> TIGSEFQNDIPDLYSVFKDYFPIGVAVDPSRLNDTDPHAQLTAKHFNMLTAENAMKPESLEPEEGRYNFEDADRIVAFAEKHGMKMRGHTLVWHQQVPDWFFLDENGNPMVDETDPKNREANREELRQRMENHIKTVAGRYKGKIYAWDVVNEVFNDDGTLRNSAWYQIIGPDYIEEALRAAHEADPNAKLFINDYNIENWSHAKTQAMYNMVRDFKERGVP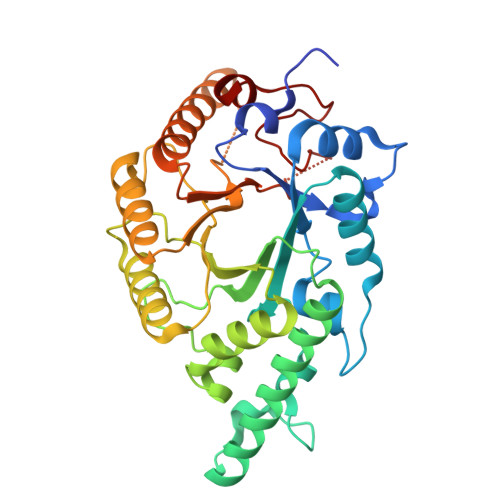VDGVGMQGHISLYYPSLEEIEKALKAFAALGVEIMITELDVNTQGDVSPDALQEQAERMRDLFELFKKHSDKITGVTFWGVADDQSWKNNFPVPGRTNAPLLFDRNYQPKPAFWAIV3-[2-(3,5-dichlorophenyl)-2-methylpropanoyl]-N-(2-{[(2Z)-2-iminoethyl]amino}-2-oxoethyl)-4-methoxybenzamide 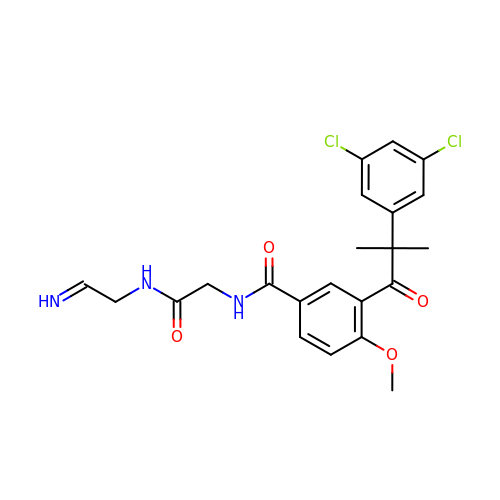| C22 H23 Cl2 N3 O4 | BXGGHAHXZXWBGP-HGBQSQDTSA-N>[2x]MVMLTLYFTPGTISVAVAIAIEEAALPYQPVRVDFATAEQTKPDYLAINPKGRVPAL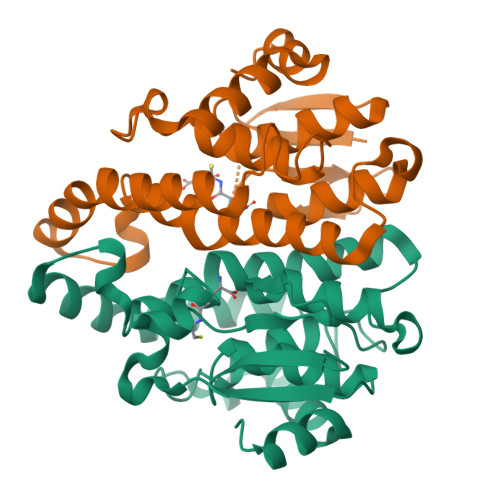RLEDDTILTETGALLDYVAAIAPKAGLVPTDPTAAAQMRSAMYYLASTMHVAHAHKMRGSRWAKQQSSFEDMTAQVPETMAACADFVESDILRGPYVLGEDFSLADPYLFVVCNWLDGDGVDTAAYPKITTFMQQMTARASVAAVKDKGMLAENLYFQ>[3x]MHLKIVCLSDEVREMYKNHKTHHEGDSGLDLFIVKDEVLKPKSTTFVKLGIK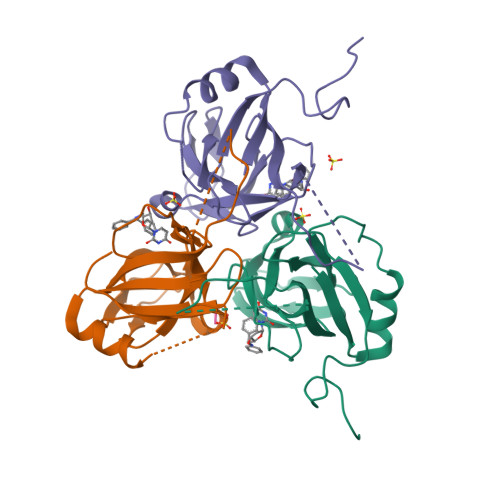AIALQYKSNYYYKCEKSENKKKDDDKSNIVNTSFLLFPRSSISKTPLRLANSIGLIDAGYRGEIIAALDNTSDQEYHIKKNDKLVQLVSFTGEPLSFELVEELDETSRGEGGFGSTSNNKYEAHHHHHH;> AHA>MADKKTDIPTLIADSTKASLQDFNHDYGKQWTFGENWSNVNTMFETYVNKYLFPKINETLLIDIALGNRFNWLAKEQDFIGQYSEEYVIMDTIPIEMNLSKSEELMLKRNYPQMATRLYGSGIVKKQKFTLNNNDVRFNFQTLGDATNYALGVLRKKISDINVQEEKEIRAMMVDYAINQLQDSNRRTASSKEDLTERVFEAILNMQNNSAKYNEVHKASGGSVGQYTTVSKLSDIAILTTDSLKSYLLDTKIANTFQMAGIDFTDHIISFDDLGGVYKTTKDVTLANEDTINYLRAFGDYQAMIGDVIPTGSVFTFNVSDLKEFKGNIEEIKPQGELFAFIFDINALKYKRNTKGMLKEPFYNGEFDEVTHWIHYYSFKAMSPFF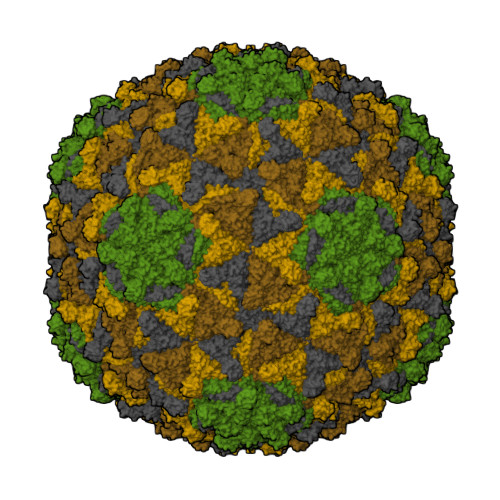NKILITEAPKEQPDAGATE[4x];>MANFDGNEMRGMTHANYEDSRLNKSRELNANMSIGTSKSEDEYGRQVHSLTKQSYSDDSVQEA[4x]The membrane-anchored SNARE (soluble N-ethylmaleimide-sensitive factor acceptor protein receptor) proteins provide the energy to drive membrane fusion in various cellular contexts, such as intracellular trafficking and exocytosis. Supercomplexes of NSF, α-SNAP, and either a syntaxin tetramer or one of two binary complexes of syntaxin—SNAP-25 reveal atomic details of SNARE processing and show how sequential ATP hydrolysis drives disassembly. NSF comprises three structured domains connected by flexible linkers—the adapter N-domain followed by the D1 and D2 AAA+ domains. Six NSF protomers come together to form the active form of the enzyme, a homo-hexamer.

A representative 21bin20S model (class #5, 3.39 Å) and ɑ-SNAP—2:1 binary SNARE subcomplex model (class #13, 3.74 Å). We again performed signal subtraction and local alignment on ɑ-SNAP—SNARE sub-complexes from all five classes with ordered spire structures (see “Methods”). This procedure produced a single ɑ-SNAP—SNARE sub-complex reconstruction with an overall resolution of 3.74 Å, sufficient to assign characteristic side chains, identify the SNAREs forming the complex and their directionality. A model composed of the ternary neuronal SNARE complex55 with synaptobrevin removed was docked into the density, preserving a distinctive kink in the peptide linker leading into the SN2 SNARE motif of SNAP-25. In place of synaptobrevin, a second syntaxin molecule was placed to complete the four-helix bundle with little deviation from its usual backbone configuration of the ternary complex. As such, the stoichiometry of the syntaxin—SNAP-25 complex observed is 2:1, the dominant species in solution. Sidechains comprising essential layers repack within the core of the complex compared to the ternary SNARE complex. For example, the ionic central layer (0 layer) is reorganized; Arg56 of synaptobrevin is replaced with a second Gln226 from the additional syntaxin molecule, which adopts an extended rotamer to mimic the arginine it replaces. Three ɑ-SNAP molecules bind the 2:1 binary SNARE complex; a flexible linker between SNAP-25 SN1 and SN2 blocks access by a fourth. The 2:1 binary SNARE complex forms a twisted, parallel ɑ-helical bundle with a series of characteristic SNARE complex layers preserved. This configuration also places the N-terminal portion of the linker, bearing cysteines often palmitoylated in vivo, near the membrane.

>[2x]MKDRTQELRTAKDSDDDDDVTVTVDRDRFMDEFFEQVEEIRGFIDKIAENVEEVKRKHSAILASPNPDEKTKEELEELMSDIKKTANKVRSKLKSIEQSIEQEEGLNRSSADLRIRKTQHSTLSRKFVEVMSEYNATQSDYRERCKGRIQRQLEITGRTTTSEELEDMLESGNPAIFASGIIMDSSISKQALSEIETRHSEIIKLENSIRELHDMFMDMAMLVESQGEMIDRIEYNVEHAVDYVERAVSDTKKAVKYQSKARRKKIM;> MGSSHHHHHHSQDPNSMAEDADMRNELEEMQRRADQLADESLESTRRMLQLVEESKDAGIRTLVMLDEQGEQLERIEEGMDQINKDMKEAEKNLTDLGKFAGLAVAPANKLKSSDAYKKAWGNNQDGVVASQPARVVDEREQMAISGGFIRRVTNDARENEMDENLEQVSGIIGNLRHMALDMGNEIDTQNRQIDRIMEKADSNKTRIDEANQRATKMLGSG;>GMDTSGKQAEAMALLAEAERKVKNSQSFFSGLFGGSSKIEEACEIYARAANMFKMAKNWSAAGNAFCQAAQLHLQLQSKHDAATCFVDAGNAFKKADPQEAINCLMRAIEIYTDMGRFTIAAKHHISIAEIYETELVDVEKAIAHYEQSADYYKGEESNSSANKCLLKVAGYAAQLEQYQKAIDIYEQVGTSAMDSPLLKYSAKDYFFKAALCHFCIDMLNAKLAVQKYEELFPAFSDSRECKLMKKLLEAHEEQNVDSYTESVKEYDSISRLDQWLTTMLLRIKKTIQGDEEDLR[3x]> DITVYNGQQKEAATAVAKAFEQETGIKVTLNSGKSEQLAGQLKEEGDKTPADVFYTEQTATFADLSEAGLLAPISEQ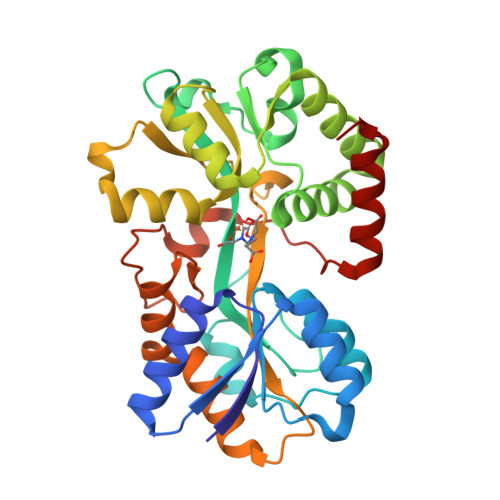TIQQTAQKGVPLAPKKDWIALSGRSRVVVYDHTKLSEKDMEKSVLDYATPKWKGKIGYVSTSGAFLEQVVALSKMKGDKVALNWLKGLKENGKLYAKNSVALQAVENGEVPAALINNYYWYNLAKEKGVENLKSRLYFVRHQDPGALVSYSGAAVLKASKNQAEAQKFVDFLASKKGQEALVAARAEYPLRADVVSPFNLEPYEKLEAPVVSATTAQDKEHAIKLIEEAGLK>MGSGLKAGDSFPSDVVFSYIPWSEDKGEITACGI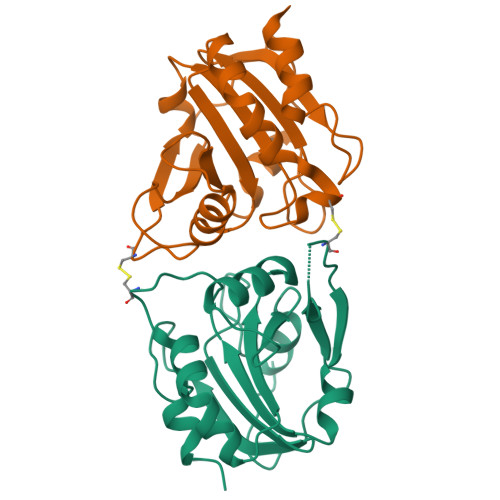PINYNASKEWADKKVILFALPGAFTPVCSARHVPEYIEKLPEIRAKGVDVVAVLAYNDAYVMSAWGKANQVTGDDILFLSDPDARFSKSIGWADEEGRTKRYALVIDHGKITYAALEPAKNHLEFSSAETVLKHLHHHHHH[2x]>MAKLETVTLGNIGKDGKQTLVLNPRGVNPTNGVASLSQAGAVPALEKRVTVSVSQPSRNRKNYKVQVKIQNPTACTANGSCDPSVTRQAYADVTFSFTQYSTDEERAFVRTELAALLASPLLIDAIDQLNPAY[180x];> MPKLPRGLRFGADNEILNDFQELWFPDLFIESSDTHPWYTLKGRVLNAHLDDRLPNVGGRQVRRTPHRVTVPIASSGLRPVTTVQYDPAALSFLLNARVDWDFGNGDSANLVINDFLFRTFAPKEFDFSNSLVPRYTQAFSAFNAKYGTMIGEGLETIKYLGLLLRRLREGYRAVKRGDLRALRRVIQSYHNGKWKPATAGNLWLEFRYGLMPLFYDIRDVMLDWQNRHDKIQRLLRFSVGHGEDYVVEFDNLYPAVAYFKLKGEITLERRHRHGISYANREGYAVFDNGSLRPVSDWKELATAFINPHEVAWELTPYSFVVDWFLNVGDILAQQGQLYHNIDIVDGFDRRDIRLKSFTIKGERNGRPVNVSASLSAVDLFYSRLHTSNLPFATLDLDTTFSSFKHVLDSIFLLTQRVKR

The coat proteins (CPs) of single-stranded RNA bacteriophages (ssRNA phages) directly assemble around the genomic RNA (gRNA) to form a near-icosahedral capsid with a single maturation protein (Mat) that binds the gRNA and interacts with the retractile pilus during infection of the host. The canonical ssRNA phage Qβ has a genomic RNA (gRNA) of 4217 nucleotides, from the 5′ to the 3′ end, encoding the maturation protein (Mat); the major coat protein (CP); the minor capsid protein A1, which is a read-through extension caused by a leaky stop codon for the major CP; and the β-subunit of the RNA-dependent RNA replicase (Rep). Like many other viruses, the CPs of ssRNA phages can also assemble into virus-like particles (VLPs), which are not infectious. Through a native infection without engineering the amino acid sequences, we found that Qβ CP can form diverse VLP capsids, including the T = 3 icosahedral, T = 4 icosahedral, prolate, oblate, and a small prolate form elongated along the 3-fold axis.

From our cryo-EM density map, we have built a complete atomic model of the Qβ virion, including the entire 4217-nucleotide long gRNA in its dominant conformation in the capsid. The gRNA folds domain by domain with the 3′ UTR (the red-ribbon portion of the model in Figure 1) packaged close to the Mat, and the 5′ UTR (the blue-ribbon in Figure 1) far away from the Mat. The RNA 5-way junction domain for Qβ, which interacts with the Mat, the internal CP dimer, and one exposed CP dimer, is determined to be the 3′ UTR of the gRNA. The last stem-loop in the entire gRNA, U1, specifically interacts with the Mat, and the stem-loop, U2, interacts with one exposed CP dimer. Unique to the Qβ is that the last stem-loop of the replicase gene, R1, specifically interacts with the internal CP dimer. The last six nucleotides of the entire gRNA, including the CCA tail, fold back to be part of the stem-loop R1 by pairing with residues 4124 to 4129. One striking feature of the gRNA fold in the Qβ is a ~200-Å long helical structure that horizontally spans the equator of the capsid when the Mat is defined as the north pole. In the complete model of the gRNA, it was determined that this long helical structure is in fact formed by shorter RNA stem-loops connected through two kissing loops (indicated by orange and red boxes in Figure 1C, zoomed-in Figure 1E). One CP dimer, at the two-fold axis on the shared edge of two hexamers, is replaced by the Mat, resulting in a total of 89 CP dimers on the capsid. For Qβ, an extra internal CP dimer interacts with stem-loop R1 of gRNA inside the capsid, still making a total of 90 CP dimers.>[4x]GSHMEQRILKFLEELGEGKATTAHDLSGKLGTPKKEINRVLYSLAKKGKLQKEAGTPP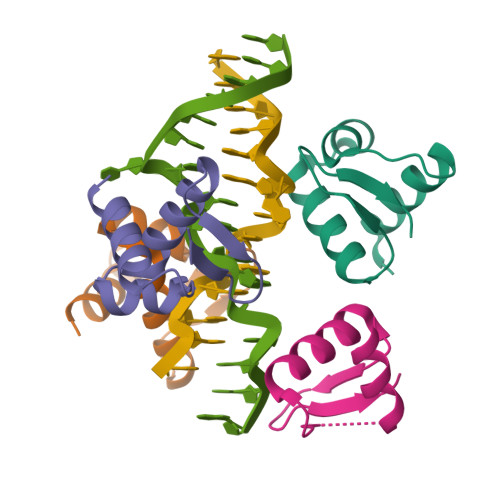LWKIA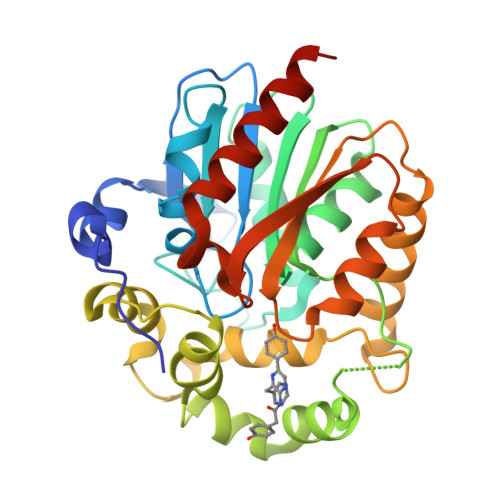>[2x]MASKVYDPEQRKRMITGPQWWARCKQMNVLDSFINYYDSEKHAENAVIFLHGNATSSYLWRHVVPHIEPVARCIIPDLIGMGKSGKSGNGSYRLLDHYKYLTAWFELLNLPKKIIFVGHDWGAALAFHYAYEHQDRIKAIVHMESVVDVIESWDEWPDIEEDIALIKSEEGEKMVLENNFFVETVLPSKIMRKLEPEEFAAYLEPFKEKGEVRRPTLSWPREIPLVKGGKPDVVQIVRNYNAYLRASDDLPKLFIESDPGFFSNAIVEGAKKFPNTEFVKVKGLHFLQEDAPDEMGKYIKSFVERVLKNEQVDHHHHHH The Eph (erythropoietin-producing hepatocyte) transmembrane receptor tyrosine kinase superfamily, with its first member identified30 years ago, contains 14 members in mammals and is the largest among all receptor tyrosine kinase families. However, the cytoplasmic portion of all 14 Eph receptors are highly similar, each containing a membrane-juxtaposing kinase domain, a protein-binding SAM domain immediately followed by a short carboxyl tail PDZ domain-binding motif (PBM). In this study, we performed systematic biochemical and structural studies of the bindings of three SAM domains, two from previously identified Eph-binding proteins (SHIP2 and Odin) and one from a new Eph-binding protein discovered in this study (SAMD5), to the SAM domains from every Eph receptor. Our study reveals that the Eph SAM domains have exquisitely specific target SAM domain-binding properties, although their overall SAM-SAM heterodimer formation modes are very similar.

Surprisingly, although the amino acid sequence of SAMD5 SAM can be aligned well (the key binding residues in particular) with the SAM domain sequences of SHIP2 and Odin (top), SAMD5 bound to EphA5-8 and EphB1-4 SAM domains with strong affinities but only weakly to EphA1/2 SAM domains. To delineate the mechanism governing the Eph/SAMD5 interaction, we solved the EphA5/SAMD5 SAM–SAM complex crystal structure at the resolution of 1.9 Å. Similar to that of EphA2/SHIP2 or EphA6/Odin, EphA5 SAM also uses its End-Helix to interact with the Mid-Loop SAMD5 SAM. The most prominent difference is that the EphA5/SAMD5 SAM-SAM does not contain the π-π stacking observed in the EphA2/SHIP2 and EphA6/Odin complexes. Instead, the EphA5/SAMD5 SAM-SAM is essentially completely mediated by charge–charge and hydrogen bonding interactions. Similar to what we observed in the EphA2/SHIP2 and EphA6/Odin structures, Gly853A5 at the beginning of α5 in EphA5 SAM is also critical for its binding to SAMD5 SAM. The backbone amine of Gly853A5 forms a strong hydrogen bond with Tyr27SAMD5 sidechain hydroxyl group. This hydrogen bond brings the α2-α3 loop of SAMD5 very close to α5 of EphA5, and the site has no room to accommodate any residues with side chains, further highlighting the importance of a Gly at this position in the Eph SAM domains. To our surprise, substitution of Tyr27SAMD5 with Phe completely eliminated SAMD5’s binding to EphA5, indicating the critical role of the Gly853A5-Tyr27SAMD5 hydrogen binding in addition to their steric role. Our crystal structure of the EphA5/SAMD5 complex can explain why SAMD5 does not bind to EphA1-4, EphA10, and EphB6.

> GPGSLGSGAYRSVGEWLEAIKMGRYTEIFMENGYSSMDAVAQVTLEDLRRLGVTLVGHQKKIMSSLQEMKVQMVNGMVPV;> GPGSMCTNIVYEWLKALQLPQYAESFVDNGYDDLEVCKQIGDPDLDAIGVLAPAHRRRILEAVHRLREQD>[2x]MGPHHHHHHLESTSLYKKAGSENLYFQGMTPGKKIPIFVDGVVLNGPQTDVKAGEKFVEEACRLIMEEVVLKATDVNEKVCEWQPPEQLRQLLDLEMRDTGESQDKLLKLCQDVIHFSVKTNHPRFFNQLYAGLDYYSLAARIITEALNPSIYTYEVSPVFLLVEEAVLKKMIECVGWKEGDGIFNPGGSVSNMCAMNLARYRHCPDIKEKGLSGLPRLILFTSAECHYSMKKAASFLGIGTQNVYFVETDGRGKMIPEDLEKQIWQARQEGAVPFLVCATSGTTVLGAFDPLDEIAEVCERHGLWLHVDASWGGSALVSRKHRRLLHGIHRADSVAWNPHKMLMAGIQCSALLVKDKSDLLKKCYSAKATYLFQQDKFYDVSYDTGDKSIQCSRRPDAFKFWMTWKALGTSGLEERVNRAFALSRYLVDEIKKREGFKLLMEPEYTNVCFWYIPPSLREMEEGPEFWRKLSLVAPAIKEKMMKKGSLMLGYQPHRGKVNFFRQVVISPQVSREDMDFLLDEIDSLGRDM

PLP-dependent decarboxylases constitute a large family of enzymes that catalyze a range of metabolic reactions. One such enzyme is glutamic acid decarboxylase-like protein 1 (GADL1), which was originally named based on its sequence homology to glutamic acid decarboxylase (GAD), which synthesizes the inhibitory neurotransmitter γ-aminobutyric acid (GABA; Fenalti et al., 2007). However, GADL1 has no reactivity towards glutamic acid and therefore is unlikely to be involved in GABA signalling. Compared with CSAD, the activity of GADL1 towards cysteine sulfinic acid (CSA) as a substrate is much lower, and GADL1 has a stronger preference for aspartate, suggesting that GADL1 may be involved in the biosynthesis of β-alanine and its peptide derivatives, such as the neuro­protectant carnosine.

In this study, we describe the crystal structure of mouse GADL1 (MmGADL1). The diffraction quality was initially poor, with diffraction limits of around 6–7 Å and highly smeared reflections. By optimizing the size, the amount of nucleation, and the general appearance of the crystals, the conditions given in Table 1 produced thin but nonfragile crystals that allowed structure refinement in two crystal forms to resolutions of 2.4 and 3.0 Å; the higher resolution data set was plagued by significant twinning and pseudotranslation. Thus, the structure of the nontwinned crystal form is discussed here; essentially all features can also be seen in the twinned crystal. For both chains, residues 11–502 could be built, with the flexible loop common to PLP-dependent decarboxylases being absent from the electron density (approximately residues 340–350). The overall fold of MmGADL1 is similar to those of CSAD and other close homologues, with a flexible loop, not defined in electron density, from the apposing monomer covering the active site, which is possibly relevant in catalysis. Importantly, a large part of the active-site cavity wall will be formed by the flexible loop in the substrate-bound state; the flexible loop is invisible in most PLP-dependent decarboxylase crystal structures, but harbours a Tyr residue that is likely to be important for catalysis. While our GADL1 preparation is enzymatically active, and the crystal is apparently fully occupied with covalently bound PLP, we cannot currently rule out the presence of PLP-deficient GADL1 in the purified SAXS sample, since crystallization might have enriched a cofactor-bound conformation of the protein. While the molecular mass calculated from the forward scattering intensity accurately matches that of a dimer, the theoretical scattering curve calculated from the crystal structure differs significantly. The shape in solution is more elongated than in the crystal.> ACYCRIPACIAGERR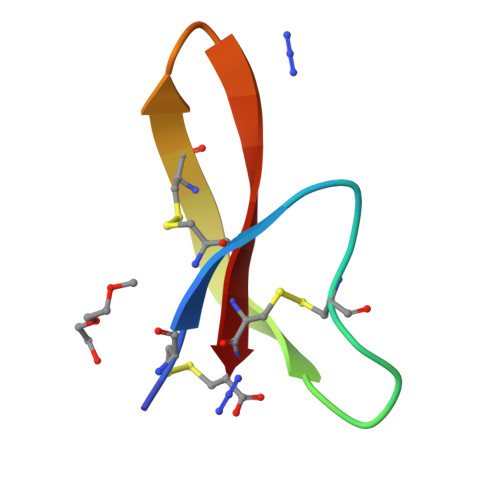AGTCIYQGRLWAFCC>MRVLGIETSCDATGIAIYDDEKGLLANQLYSQVKLHADYGGVVPELASRDHVRKTVPLIQAALKESGLTAKDIDAVAYTAGPGLVGALLVGATVGRSLAFAWDVPAIPVHHMEGHLLAPMLEDNPPEFPFVALLVSGGHTQLISVTGIGQYELLGESIDDAAGEAFDKTAKLLGLDYPGGPLLSKMAAQGTAGRFVFPRPMTDRPGLDFSFSGLKTFAANTIRDNGTDDQTRADIARAFEDAVVDTLMIKCKRALDQTGFKRLVMAGGVSANRTLRAKLAEMMKKRRGEVFYARPEFCTDNGAMIAYAGMVRFKAGATADLGVSVRPRWP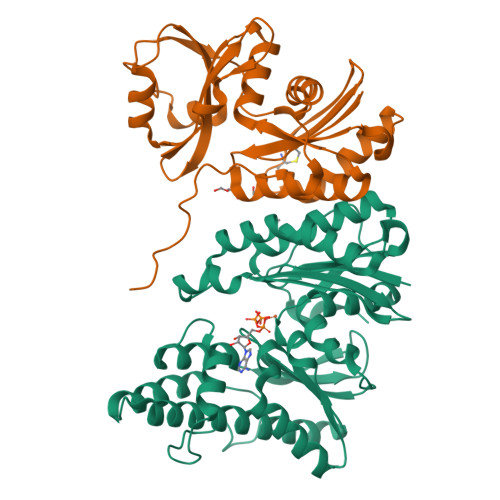LAELPAAHHHHHH[2x];>MRILAIDTATEACSVALWNDGTVNAHFELCPREHTQRILPMVQDILTTSGTSLTDINALAYGRGPGSFTGVRIGIGIAQGLALGAELPMIGVSTLMTMAQGAWRKNGATRVLAAIDARMGEVYWAEYQRDENGIWHGEETEAVLKPEIVHERMQQLSGEWVTVGTGWQAWPDLGKESGLVLRDGEVLLPAAEDMLPIACQMFAEGKTVAVEHAEPVYLRNNVAWKKLPGKEHHHHHH[2x]> MAPSRLCVYCADVCPDRLRCAAWLLATGIFLLLAGCSEAKAPTALERVQKEGVLRVITRNSPATYFQDRNGETGFEYELAKRFAERLGVELKIETADNLDDLYAQLSREGG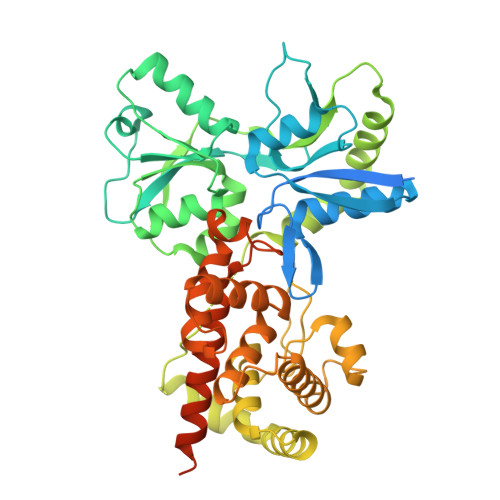PALAAAGLTPGREDDASVRYSHTYLDVTPQIIYRNGQQRPTRPEDLVGKRIMVLKGSSHAEQLAELKKQYPPLKYEESDAVEVVDLLRMVDVGDIDLTLVDSNELAMNQVYFPNVRVAFDFGEARGLAWALPGGDDDSLMNEVNAFLDQAKKEGLLQRLKDRYYGHVDVLGYVGAYTFTQHLQQRLPRYESHFKQSGKQKDTDWRLLAAIGYQESLWQPGATSKTGVRGLMMLTNRTAQAMGVSNRLDPKQSIQGGSKYFVQIRSELPESIKEPDRSWFALAAYNIGGAHLEDARKMAEKEGLNPNKWLDVKKMLPRLAQKQWYAKTRYGYARGGETVHFVQNVRRYYDILTWVTQPQMEGSQIAESGLHLPGVNKTRPEEDSGDEKL> MYEGRWKMVNQIKQDVQNDIELILRQMNERIHAMKKKKYNELKGKIKQKCIDLLIDYAKQKIGKKNKIKKEGNNIRHNKQKKLKNIQKKIFKIISTRMLQTTLSAFRPRGSNVTGKVALATLGALTGYGAFYHYNQYLNLSARWQQIQENIAKDQPFDVDGFDAKVYPWVRENNVNDWEYKLVKMRGYFKDQRFFVRRKRDGKEGFLVF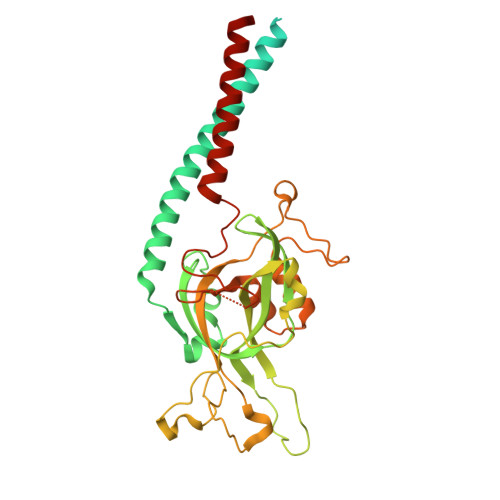APFVTAVERVNHRLKQKDLLPVEYSVFVNLGWVPVENKKDVELGGEVCPPMDAPTDSTLFVNDTFTGFNPDPANPEDTEQVTLTEITGIVRRGEQQDILARRRNWNKEGIYNWVDLDYMGKIFRLFNLDAINTAYIERVVPSFEEGEEGLYPIPATKDTFERPLNTPERHSTFFNFYAATSALSFISMLLLRR> GPLGSMEAARPPPTAGKFVVVGGGIA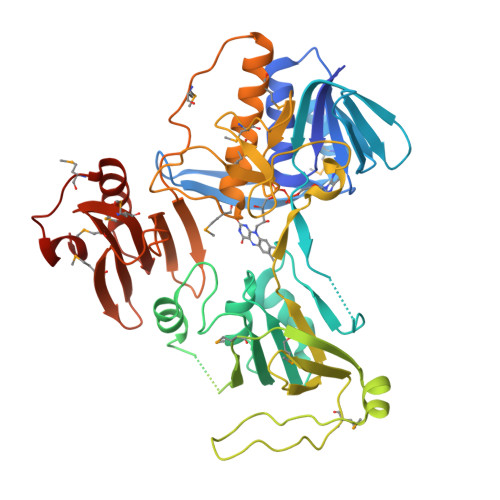GVTCAEQLATHFPSEDILLVTASPVIKAVTNFKQISKILEEFDVEEQSSTMLGKRFPNIKVIESGVKQLKSEEHCIVTEDGNQHVYKKLCLCAGAKPKLICEGNPYVLGIRDTDSAQEFQKQLTKAKRIMIIGNGGIALELVYEIEGCEVIWAIKDKAIGNTFFDAGAAEFLTSKLIAEKSEAKIAHKRTRYTTEGRKKEARSKSKADNVGSALGPDWHEGLNLKGTKEFSHKIHLETMCEVKKIYLQDEFRILKKKSFTFPRDHKSVTADTEMWPVYVELTNEKIYGCDFIVSATGVTPNVEPFLHGNSFDLGEDGGLKVDDHMHTSLPDIYAAGDICTTSWQLSPVWQQMRLWTQARQMGWYAAKCMAAASSGDSIDMDFSFELFAHVTKFFNYKVVLLGKYNAQGLGSDHELMLRCTKGREYIKVVMQNGRMMGAVLIGETDLEETFENLILNQMNLSSYGEDLLDPNIDIEDYFD>[4x]ADCPPGWSSYDLYCYQGFNGPQTWDDAERFCTEQAKGGHLVSISDSGEADFVGQLITQNISRPEYYVWTGLRDRRSEQQCNPEWNDGSSIIYTNWDSGESEMCQAFSRWTNFREWMNTNCQQKNPFVCKFPPA;>DCPSGWSSYDGHCYQVFSDLKNWDDAESFCSGQHEGSRLASIHSREEEAFVGKMASRTLKYTSMWLGLNNPWKECKWEWSDDTRLDYKVWTRRPYCTVMVVKTDRIFWFNRGCEKSVSFVCKFKAYSEDAAE[4x]

In this study, we demonstrated the isolation, purification, and characterization of a novel snake venom protein with anti-angiogenic and anti-inflammatory activity, ZK002. In the first part of this paper, we described the isolation and purification of ZK002 and its identification as a 30 kDa heterodimer of α and β peptide chains of the snaclec class of proteins. Snaclecs are approximately 30 kDa in mass with heterodimeric structures comprised of homologous α and β subunits linked by a disulfide bond. Our results showed that ZK002 exhibited potent anti-angiogenic activity, with inhibition of tube formation, cell migration, and cell invasion in VEGF-induced HUVECs, and significant anti-angiogenic activity in multiple in vivo models.

The purified protein showed a molecular mass of 30 kDa, and two distinct peaks with a molecular mass of 15 kDa (α subunit) and 16 kDa (β subunit), results in line with our previous SDS-PAGE experiments indicating that ZK002 is a disulfide-linked heterodimer. Database search showed the sequence of the β-chain was a complete match to an existing snake venom C-type lectin protein (snaclec) of D. actus (UniProtKB: Q8JIV8). The sequence with highest similarity to the ZK002 α-chain was Snaclec stejaggregin-A subunit alpha (UniProtKB: Q71RQ1.1), to which it shared 76% identity, thus indicating that the α-chain was a novel sequence. NCBI Conserved Domain Database analysis indicated that both ZK002 α and β possessed C-type lectin-like domains, a prototypical domain featured in snaclecs. The structure of ZK002 was determined via X-ray crystallography to a resolution of 2.1 Å. In agreement with the mass spectrometry results above, ZK002 exists as an αβ heterodimer. In line with previous reports on snaclecs, the structure of both α and β chain subunits of ZK002 comprised two β-sheets consisting of the β strands β0–β1–β5 and β2–β3–β4, connected by two orthogonally orientated α-helices, and a long loop was seen between β2 and β3 strands. Further, disulphide bridges between cysteine residues were seen between β0 and β1, α1 and β5, β3 and the loop region of β5, and between the two loop regions of the heterodimers. The asymmetric crystallographic unit was made up of a tetramer of αβ heterodimers. Taken together, the sequence and structure of ZK002 were strongly consistent with that of the snaclecs class of proteins.> GSHMRIPATIKKKMALPPATPVFTG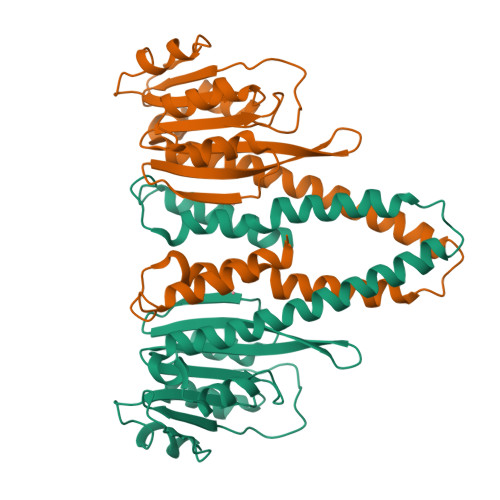EKKVEETKITAAIYDEKSVEFKELEVGELESVVRSALALNKKLWIDVVGVHDESLIAKICEFLGIHPLAAEDILNTAQRVKIEDYDDHLFLVLKILLYNETLEIDQLSLVLKKNLVATFEEREYWILDSIRSRLKSGGRMRKLAGDYLAYTILDAVVDSYFEALLKISDEIEVLEDEVVSGDSTLIGKIHSLKREILAFRNAVWPLRDVLSFFTRVEHELIGEEVKVYYRDVYDHAVRLME>HMRQRHILFANVQGHGHVYPSLGLVSELARRGHRITYVTTPLFADEVKAAGAEVVLYKSEFDTFHVPEVVKQEDAETQLHLVYVRENVAILRAAEEALGDNPPDLVVYDVFPFIAGRLLAARWDRPAVRLTGGFAANEHYSLFKELWKSNGQRHPADVEAVHSVLVDLLGKYGVDTPVKEYWDEIEGLTIVFLPKSFQPFAETFDERFAFVGPTLTGRDGQPGWQPPRPDAPVLLVSLGNQFNEHPEFFRACAQAFADTPWHVVMAIGGFLDPAVLGPLPPNVEAHQWIPFHSVLAHARACLTHGTTGAVLEAFAAGVPLVLVPHFATEAAPSAERVIELGLGSVLRPDQLEPASIREAVER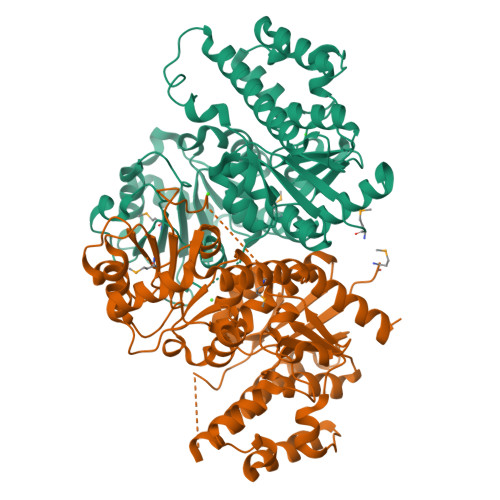LAADSAVRERVRRMQRDILSSGGPARAADEVEAYLGRVAP[2x]>MHHHHHHENLYFQGPKPPIDLVVTETTATSVTLTWDSGNSEPVTYYGIQYRAAGTEGPFQEVDGVATTRYSIGGLSPFSEYAFRVLAVNSIGRGPPSEAVRARTGEQAPSSPPRRVQARMLSASTMLVQWEPPEEPNGLVRGYRVYYTPDSRRPPNAWHKHNTDA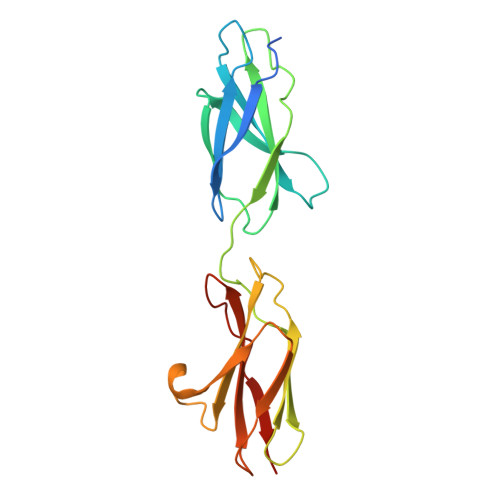GLLTTVGSLLPGITYSLRVLAFTAVGDGPPSPTIQVKTQQGVP[2x]> GYSDRVRSITLGNSTITTQECANVVVGYGEWPEYLSDNEATAEDQPTQPDVATCRFYTLDSVQWENGSPGWWWKFPDALRDMGLFGQNMYYHYLGRAGYTIHV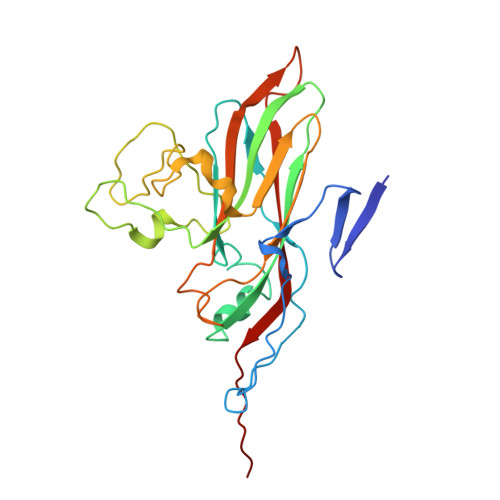QCNASKFHQGCILVVCVPEAEMGSAQTSGVVNYEHISKGEIASRFTTTTTAEDHGVQAAVWNAGMGVGVGNLTIFPHQWINLRTNNSATIVMPYVNSVPMDNMYRHHNFTLMIIPFVPLDFSAGASTYVPITVTVAPMCAEYNGLRLAGHQ[(2~{R},3~{S},4~{R},5~{R})-5-(6-aminopurin-9-yl)-3,4-bis(oxidanyl)oxolan-2-yl]methyl 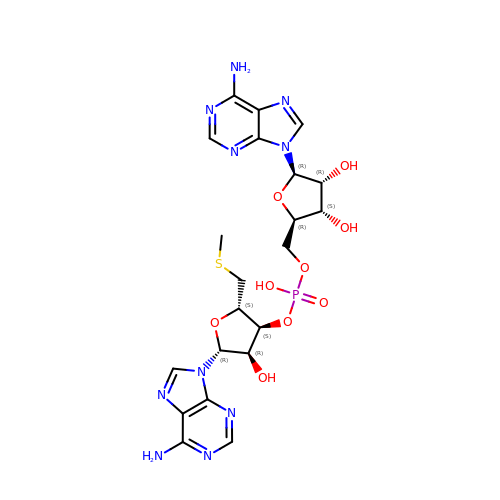[(2~{S},3~{S},4~{R},5~{R})-5-(6-aminopurin-9-yl)-2-(methylsulfanylmethyl)-4-oxidanyl-oxolan-3-yl] hydrogen phosphate | C21 H27 N10 O9 P S | NNWVUANIXUHJMY-NAGRZYTCSA-N(2R,5R)-2,5-diamino-2,5-bis(4-aminobutyl)hexanedioic acid | C14 H30 N4 O4 | 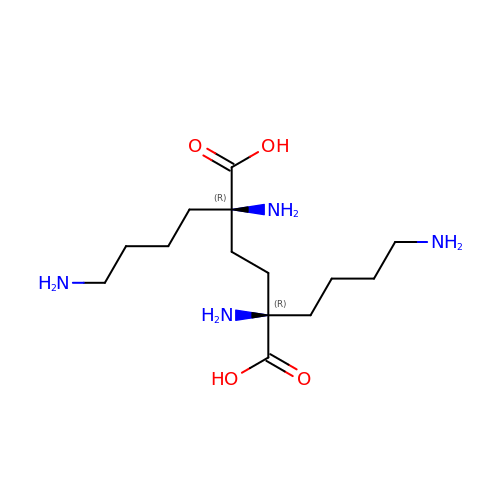XYUHPPVEDOOPDE-ZIAGYGMSSA-N First, DegP is an allosteric protease, whose activity is carefully regulated, and a hyperactive DegP variant kills bacteria. Second, because DegP is an inherently promiscuous protease that degrades misfolded proteins, over-activated DegP may destroy various proteins that mediate essential processes in the bacterial envelope, such as cell wall maintenance, membrane construction, or cell division. Previous report showed that substrate binding accompanies several allosteric behaviors of DegP: proteolytic activation, assembly of cage-like proteolytic chamber and positively cooperative binding of a substrate. DegP mainly degrades misfolded proteins, but its over-activation by the tripodal compounds triggers excessive degradation of newly synthesized proteins and leads to bacterial death.

Interestingly, activation was observed with TMB_CYRKL and TMB_CKYRKL, but not with TMB_CRKL or TMB_CKL. In particular, TMB_CYRKL increased the cleavage rate by at least ten times more than Lpp+Leu and TMB_CKYRKL. The concentration-dependent activation and inhibition suggest that the tripodal compounds also bind to the active site of DegP. Alanine substitution of each residue of the pentapeptide (CYRKL) revealed that tyrosine is most important for activation. Aside from the allosteric activation, we also analyzed the effects of the two compounds on assembly of cages and cooperative binding of a substrate, and found that both TMB_CYRKL and TMB_CYYKI assemble DegP cages, but that they differently affect the binding of model substrates. Overall DegP structures were almost identical to that of the dodecameric DegP with an active conformation (rmsd 0.697 Å and 0.986 Å, respectively, for 2309 Cα atoms in six DegP subunits). Additional electron density maps were found at positions where two degrons of 18–58 are present in the dodecamer model. Because CYRKL and CYYKI have hydrophobic C-terminal residues that can occupy both the S1 pocket of the active site and the hydrophobic pocket of PDZ1, we believe that these peptides are located in the two substrate-binding sites in the same fashion as two degrons of 18–58. Taken together, the crystal structures suggest that the tripodal compounds mainly bind to the substrate-binding sites of DegP.

>[6x]AQQMPSLAPMLEKVMPSVVSINVEGSTTVNTPRMPRNFQQFFGDDSPFCQEGSPFQSSPFCQGGQGGNGGGQQQKFMALGSGVIIDADKGYVVTNNHVVDNATVIKVQLSDGRKFDAKMVGKDPRSDIALIQIQNPKNLTAIKMADSDALRVGDYTVAIGNPFGLGETVTSGIVSALGRSGLNAENYENFIQTDAAINRGNAGGALVNLNGELIGINTAILAPDGGNIGIGFAIPSNMVKNLTSQMVEYGQVKRGELGIMGTELNSELAKAMKVDAQRGAFVSQVLPNSSAAKAGIKAGDVITSLNGKPISSFAALRAQVGTMPVGSKLTLGLLRDGKQVNVNLELQQSSQNQVDSSSIFNGIEGAEMSNKGKDQGVVVNNVKTGTPAAQIGLKKGDVIIGANQQAVKNIAELRKVLDSKPSVLALNIQRGDSTIYLLMQ;>[12x]CYRKL>[14x]MM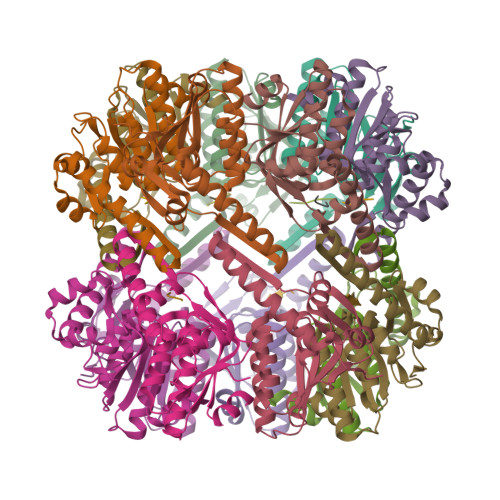GYIPYVIENTDRGERSYDIYSRLLKDRIVLLSGEINDSVASSIVAQLLFLEAEDPEKDIGLYINSPGGVITSGLSIYDTMNFIRPDVSTICIGQAASMGAFLLSCGAKGKRFSLPHSRIMIHQPLGGAQGQASDIEIISNEILRLKGLMNSILAQNSGQSLEQIAKDTDRDFYMSAKEAKEYGLIDKVLQKNVK;>[8x]NVLGFTQ> SNAAIASEFSSLPSYAAFATAQEAYEQAVANGDSEVVLKKLKKSLNVAKSEFDRDAAMQRKLEKMADQAMTQMYKQARSEDKRAKVTSAMQTMLFTMLRKLDNDALNNIINNARDGCVPLNII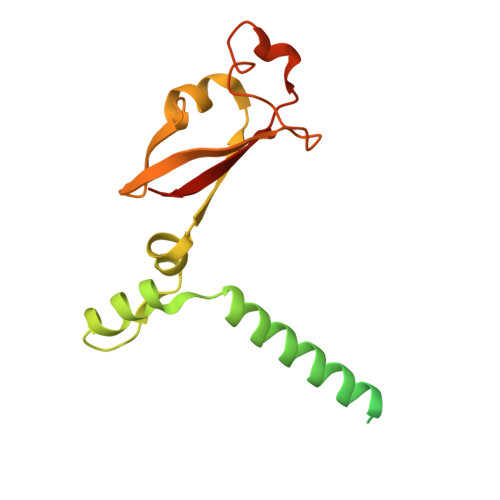PLTTAAKLMVVIPDYNTYKNTCDGTTFTYASALWEIQQVVDADSKIVQLSEISMDNSPNLAWPLIVTALRANSAVKLQ The fungal Bromodomain and Extra‐Terminal (BET) protein Bdf1 is a potential antifungal target against invasive fungal infections. One attractive target is the fungal BET protein Bdf1, a global transcriptional regulator. BET proteins bind chromatin through their two bromodomains (BDs), BD1 and BD2, which specifically recognize histones acetylated on lysines. We show that Bdf1 is essential in C. glabrata, and that inactivation of both Bdf1 BDs induces lethality.

We used a peptide array comprising histone sequences with diverse post‐translational modifications to probe the ligand selectivity of C. glabrata Bdf1 (CgBdf1) BD1 and BD2 (CgBD1 and CgBD2). Like other BET BDs, the two CgBDs displayed weak binding to mono‐acetylated peptides, enhanced binding to di‐ and tri‐acetylated peptides, and strongest binding to a tetra‐acetylated H4 peptide (H4ac4; acetylated on K5, K8, K12 and K16). Substituting a conserved tyrosine implicated in acetyllysine recognition by a phenylalanine (“Y/F” mutations Y166F and Y343F) abolished the interaction with acetylated peptides on the array and in pull‐down assays, demonstrating binding specificity. Crystal structures of CgBD1 and CgBD2 confirmed the expected BD fold (comprising helices Z, A, B and C), allowed comparison with human BET and C. albicans Bdf1 (CaBdf1) BD structures, and revealed details of the ligand binding pockets defined by the ZA and BC loops, including six structurally conserved water molecules. CgBD2 undergoes a minor conformational change to accommodate IBET‐151: in unbound CgBD2, the side chain of “YPF‐shelf” residue Tyr327 adopts a gauche minus (g−) conformation, stabilized by a sulfur‐π interaction with residue Met395, whereas, in the complex, Tyr327 adopts the trans conformation to avoid a steric clash with I‐BET151, thereby widening the ligand binding pocket.

>[7x]AMGQRAMKFCQGVVRELMSKKYASFNYPFLEPVDPVALNCPTYFDYVKEPMDLGTVSKKLSNWEYENLDQAEHDIRLIFQNCYAFNPDGTIVNMMGHRLEDIFNTKWADRPLYSDVES>[2x]FKRFSKKKEAPEDPKNLINIDKPIKELPASIAIPKEKPLTGEQQKMYDEVLKHFSNPDLKVYTSEKNKSEDDLKPLEEEEKAWLTRECFLRYLRATKWVLKDCIDRITMTLAWRREFGISHLGEEHGDKITADLVAVENESGKQVILGYENDARP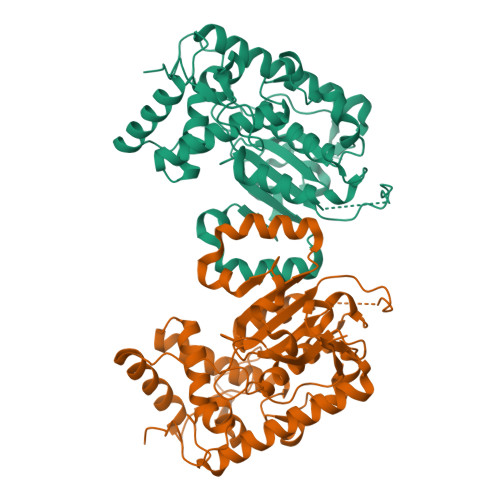ILYLKPGRQNTKTSHRQVQHLVFMLERVIDFMPAGQDSLALLIDFKDYPDVPKVPGNSKIPPIGVGKEVLHILQTHYPERLGKALLTNIPWLAWTFLKLIHPFIDPLTREKLVFDEPFVKYVPKNELDSLYGGDLKFKYNHDVYWPALVETAREKRDHYFKRFQSFGGIVGLSEVDLRGTHEKLLYPVKSESSTV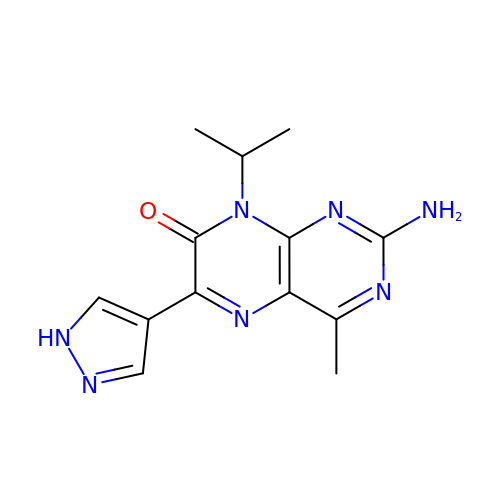2-amino-4-methyl-8-(1-methylethyl)-6-(1H-pyrazol-4-yl)pteridin-7(8H)-one | C13 H15 N7 O | YIFGKPFEGAUADP-UHFFFAOYSA-N The naphthyridine carbamate dimer (NCD) is a small molecule that recognizes disease-related RNA containing UGGAA repeats associated with spinocerebellar ataxia type 31 (SCA 31) and alleviates the disease phenotype in vitro and in vivo. SCA 31 is an autosomal spinocerebellar neurodegenerative disorder. It is caused by abnormally repeated 5′-UGGAA-3′/5′-UGGAA-3′ RNA pentads, which sequester many cellular proteins by forming toxic nuclear foci. Each of the oligomers formed self-complementary duplex: ROG1 (GGCACUGGAAGUGC)2 and ROG2 (GGCACUGGAAGUGCC)2; containing the 5′-UGGAA-3′/5′-UGGAA-3′ pentad motif selectively recognized by NCD. We crystallized two RNA–ligand complexes: ROG1–NCD (1.50 Å resolution) and ROG2–NCD (2.55 Å resolution) and one unliganded duplex of ROG2 oligomer (2.79 Å).

In both liganded structures, the asymmetric unit contained one RNA duplex consisting of chains A and B. The superposition of the ROG1–NCD and ROG2–NCD models showed similarity, with an r.m.s.d (root mean square deviation) value of 0.8 Å. The pentad motif bound two NCD molecules that interacted with all four guanosine residues. As a result, six base pairs were formed: two 6U–10A pairs and four pseudo-canonical naphthyridine-guanine pairs. The 9A residues were flipped out and engaged in crystal lattice contacts with symmetry-related RNA molecules. The NCD molecules were located in the minor groove of the 5′-UGGAA-3′/5′-UGGAA-3′ motif. Each ligand bound two guanosine residues located on the same RNA strand, forming identical pseudo-canonical NCD-G pairs. In ROG2 and ROG2–NCD models, lattice contacts were formed by stacking interactions between symmetry-related duplexes, resulting in the formation of pseudo-continuous helices. In the liganded models, the pentad loop was unwound, resulting in loss of helicity. Both 9A residues were flipped out, while guanosines interacting with the NCD ligands formed a double-stranded stem resembling the Z-RNA like structure. However, although the pentad motif resembled many structural features of the Z-RNA form, the structure remained right-handed, as in A-RNA.

>GGCACUGGAAGUGCC[2x]>[2x]GSGSPLAQQI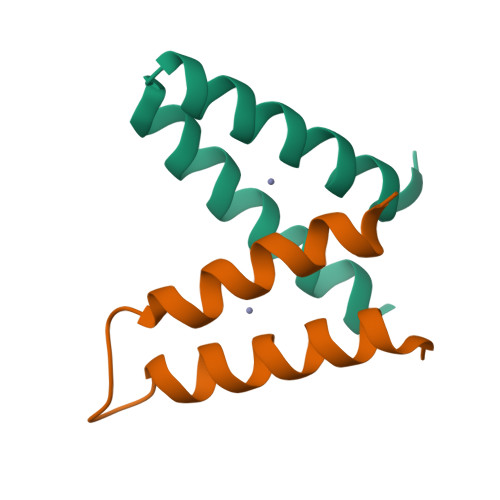KNIESFIHQAKAAGRMDEVRTLQENLHQLMHEYFQQSD> GSAEEWYFGKITRRESEALLLNPENPRGTFLVRESETTKGAYCLSVSDFDNAKGLNVKHYKIRK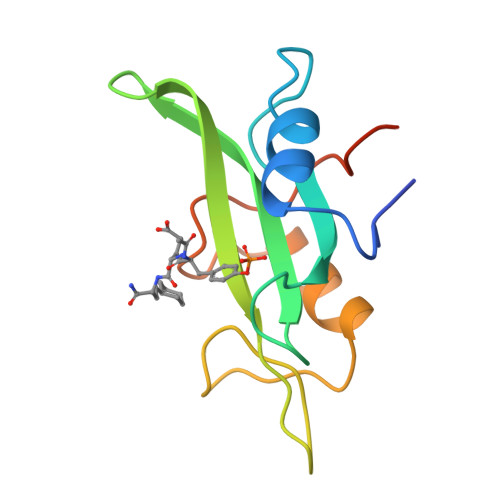LDSGGFYITSRTQFSSLQQLVAYYSKHADGLCHRLTNVCPTSKEFIVTD> SVALVPHVGMGLETRTETWMSSEGAWKHAQRIETWVLRHPG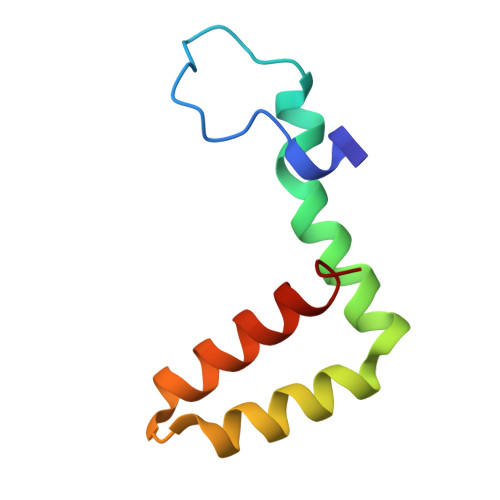FTIMAAILAYTIGTTYFQRVLIFILLTAVAPSMT BusR is a member of a yet structurally uncharacterized subfamily of the GntR family of transcription factors that downregulates transcription of the genes for the BusA (OpuA) glycine-betaine transporter upon c-di-AMP binding. BusR satisfies the overall domain architecture of the GntR family with its N-terminal winged helix-turn-helix motif (wHTH) and a C-terminal effector binding motif, an RCK_C domain (regulator of K+ conductance). Our structural data, supported by biochemical and biophysical data, reveal that BusR utilizes a unique domain assembly with a tetrameric coiled-coil in between the binding platforms, serving as a molecular ruler to specifically recognize a 22 bp separated bipartite binding motif. Binding of c-di-AMP to BusR induces a shift in equilibrium from an inactivated towards an activated state that allows BusR to bind the target DNA, leading to transcriptional repression.

We purified and crystallized a construct comprising only the RCK_C domain (Leu135 to end) and solved its ligand-free and c-di-AMP bound structure to 1 and 1.2 Å resolution, respectively. The crystal of the RCK_C domain in the c-di-AMP bound state contains the physiological dimer in the asymmetric unit with one moiety of c-di-AMP bound. The c-di-AMP binding pocket is localized in the cleft between αR1 of the two RCK_C subunits in a conserved hydrophobic and narrow pocket formed by residues Ile153, Gly154, Val158, Ala164, Thr165, Ile166, Pro181 and the main chain of Trp159 and Gly180. Residues Asn157 and His160 form a polar rim around the pocket. The high-resolution structure of the RCK_C domain explains very well the high specificity of BusR for c-di-AMP and how it discriminates its ligand even from structurally closely related molecules such as its linearized variant 5′-pApA, or c-di-GMP. The adenine base, especially its amino group forms hydrogen bonds to the peptide backbone of Ile166 while Ala164 at the same time prevents a larger group at C2 of the adenine base, thus preventing c-di-GMP from binding. The 2′-OH group of the ribose is coordinated via a hydrogen bond by Asp157 and the phosphate group forms a hydrogen bond with His160. The individual monomers are identical and the resulting assembly is symmetric, therefore all protein-ligand interactions are mirrored on the opposite site of c-di-AMP. The apo and c-di-AMP bound crystal structure of the RCK_C domain show that c-di-AMP binding induces a subtle rotation of the RCK_C domains that results in a widening of the binding pocket. This movement pushes residues Pro179, Gly180, Pro181 and Phe182 (chain A) further out in respect to Trp159 (chain B) of the opposing chain.

>GPLAPYEIIVSEDSEHLGKSIGELNVWHQTGATIVAIEHEGKFIVSPGPFSVIEQGDHIFFVGDEDVYARMKTYFNLRMGL[2x]>[6x]MSKSDVFHLGLTKNDLQGATLAIVPGDPDRVEKIAALMDKPVKLASHREFTTWRAELDGKPVIVCSTGIGGPSTSIAVEELAQLGIRTFLRIGTTGAIQPHINVGDVLVTTASVRLDGASLHFAPLEFPAVADFECTTALVEAAKSIGATTHVGVTASSDTFYPGQERYDTYSGRVVRHFKGSMEEWQAMGVM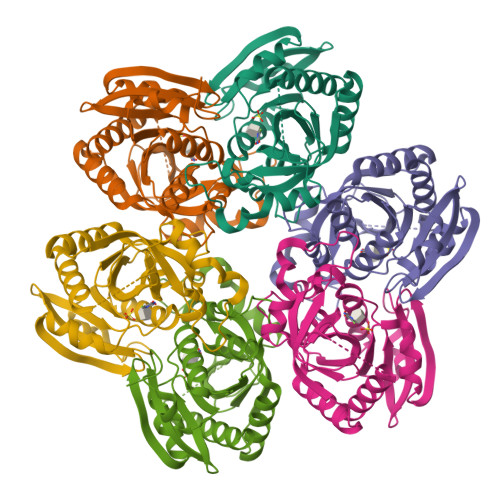NYEMESATLLTMCASQGLRAGMVAGVIVNRTQQEIPNAETMKQTESHAVKIVVEAARRLL>[2x]SSNDNIELVDFQNIMFYGDAEVGDNQQPFTFILDTGSANLWVPSVKCTTAGCLTKHLYDSSKSRTYEKDGTKVEMNYVSGTVSGFFSKDLVTVGNLSLPYKFIEVIDTNGFEPTYTASTFDGILGLGWKDLSIGSVDPIVVELKNQNKIENALFTFYLPVHDKHTGFLTIGGIEERFYEGPLTYEKLNHDLYWQITLDAHV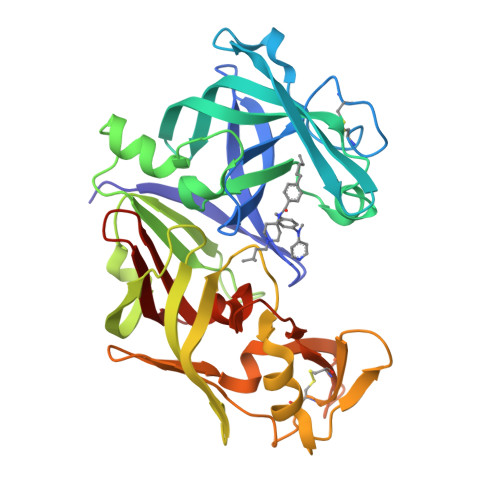GNIMLEKANCIVDSGTSAITVPTDFLNKMLQNLDVIKVPFLPFYVTLCNNSKLPTFEFTSENGKYTLEPEYYLQHIEDVGPGLCMLNIIGLDFPVPTFILGDPFMRKYFTVFDYDNHSVGIALAKKNL>[2x]MRIIMPVEFSRIVRDVERLIAVEKYSLQGVVDGDKLLVVGFSEGSVNAYLYDGGETVKLNREPINSVLDPHYGVGRVILVRDVSKGAEQHALFKVNTSRPGEEQRLEAVKPMRILSGVDTGEAVVFTGATEDRVALYALDGGGLRELARLPGFGFVSDIR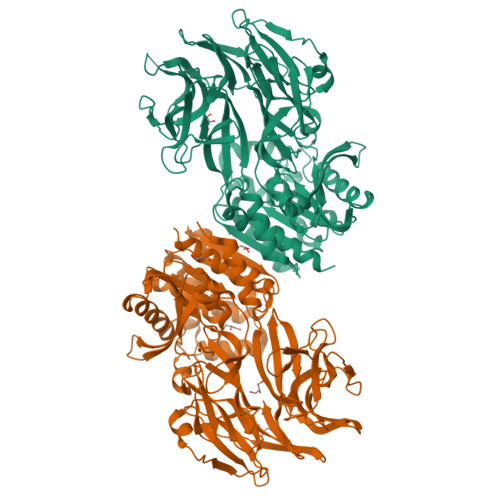GDLIAGLGFFGGGRVSLFTSNLSSGGLRVFDSGEGSFSSASISPGMKVTAGLETAREARLVTVDPRDGSVEDLELPSKDFSSYRPTAITWLGYLPDGRLAVVARREGRSAVFIDGERVEAPQGNHGRVVLWRGKLVTSHTSLSTPPRIVSLPSGEPLLEGGLPEDLRRSIAGSRLVWVESFDGSRVPTYVLESGRAPTPGPTVVLVHGGPFAEDSDSWDTFAASLAAAGFHVVMPNYRGSTGYGEEWRLKIIGDPCGGELEDVSAAARWARESGLASELYIMGYSYGGYMTLCALTMKPGLFKAGVAGASVVDWEEMYELSDAAFRNFIEQLTGGSREIMRSRSPINHVDRIKEPLALIHPQNASRTPLKPLLRLMGELLARGKTFEAHIIPDAGHAINTMEDAVKILLPAVFFLATQRERR>[12x]TRDQNGTWEMESNENFEGYMKALDIDFHTRKIAVRLTQTKVIDQDGDNFKDKTTSTFRNYDVDFTVGVEFDEYTKSLDNRHVKALVTWEG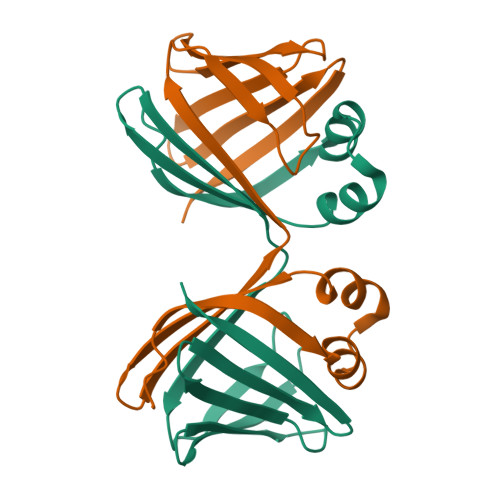DVLVCVQKGEKENRGWKKWIEGDKLYLELTCGDQVCRQVFKKK> GPHMLKIADQSVDLNLKLMKWRILPDLNLDIIKNTKVLLLGAGTLGCYVSRALIAWGVRKITFVDNGTVSYSNPVRQALYNFEDCGKPKAELAAASLKRIFPLMDATGVKLSIPMIGHKLVNEEAQHKDFDRLRALIKEHDIIFLLVDSRESRWLPSLLSNIENKTVINAALGFDSYLVMRHGNRDEQSSKQLGCYFCHDVVAPTDSLTDRTLDQ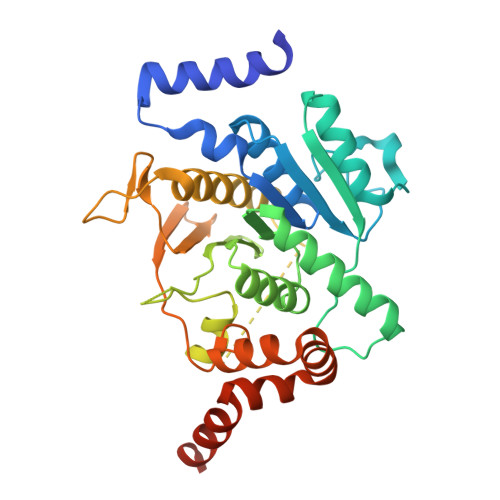MCTVTRPGVAMMASSLAVELMTSLLQTKYSGSETTVLGDIPHQIRGFLHNFSILKLETPAYEHCPACSPKVIEAFTDLGWEFVKKALEHPLYLEEISGLSVIKQEVERLGNDVFEWEDDESDEIA> GGGGGACGGUCCGGCGACCAGCGGGUCUCUAAAACCUAGCCA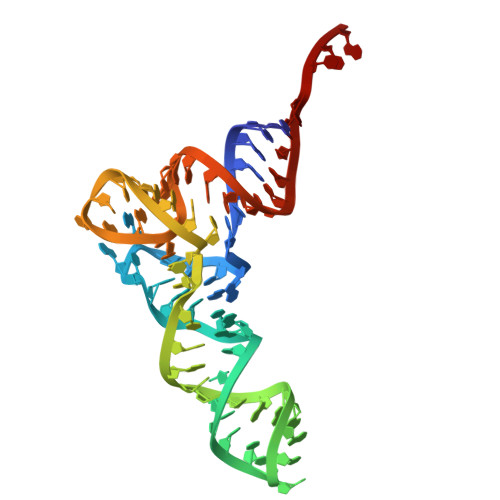GCGGGGUUCGACGCCCCGGUCUCUCGCCA In this study, we identified four enzymes (two GH183 endo-d-arabinanases, GH172 exo-α-d-arabinofuranosidase, and GH116 exo-β-d-arabinofuranosidase) from Microbacterium arabinogalactanolyticum. These enzymes completely degraded the complex d-arabinan core structure of lipoarabinomannan and arabinogalactan in a concerted manner. Furthermore, through biochemical characterization using synthetic substrates and X-ray crystallography, we elucidated the mechanisms of substrate recognition and anomer-retaining hydrolysis for the α- and β-d-arabinofuranosidic bonds in both endo- and exo-mode reactions. We propose a d-arabinan-degrading pathway for Mi. arabinogalactanolyticum based on its gene cluster and four characterized enzymes.

ExoMA1 had an optimal pH of 5.5 and was specific for the α-d-Araf bond. The crystal structure of ExoMA1 was determined at 2.42 Å resolution in the apo form. ExoMA1 assembles four trimers to form a dodecamer. ExoMA1 monomer has a double jelly-roll fold, which was found only in GH172 among over 160 GH families. The active site is located at the interface between the two subunits of the basal trimer. One phosphate molecule per monomer was bound to the interface of ExoMA1, which is responsible for dodecamer assembly. Other GH172 members (αFFase1 and a hypothetical protein BACUNI_000161 from Bacteroides uniformis) had been shown to form distinct quaternary structures depending on the mode of contact of the basal trimer. The dodecameric structure of ExoMA1 is formed by the interactions of four loops above the double jelly-roll fold, whereas the C-terminal helix is mainly involved in the hexamer (dimer of trimers) interactions in αFFase1 and BACUNI_000161. The corresponding residue in ExoMA1 is Asn253, and its side chain blocks α-d-Fruf binding, making the enzyme specific for α-d-Araf. ExoMA1 has a unique dodecameric structure compared to the various quaternary structures of the GH172 enzymes. ExoMA1 hydrolyzed the terminal α-d-Araf structures of arabinooligosaccharides released by EndoMA1 and EndoMA2 but did not act on MsLAM, A22BβT, and A7Bβ.

>MPDLNSIAALRQVQTRSISPENFDGTAGGGGRATEGTGADCARDLGPGWKISPSVDIKAGETFELASIEGAGKITHIWITTHTDNWRTLILRAFWDGADEPAVEVPYGDFFCNGWGVFAQVNSQAIAANPHGGFNSYWPMPFRDGARLTIENTSVVDVRVYYQVTYEIGGDHSNDAYFHAQWRRSNPLEELTPHVILEGIEGEGHYVGTYIAWGVNSNGWWGEGEIKFYLDDDTDHPTICGTGTEDYFGGAWNFDIPGKGYTEFSTPYLGMPQVIRPDGLYVSQQRFGMYRWHLQDPIHFATGIPKVDIQALGWRSGWRYLPLRDDIASTAMFYLDRPTARRPKSPSADDMEVHLGTAPVPDLGATPPRVLEHHHHHH[12x]> MACPLEKALDVMVSTFHKYSGKEGDKFKLNKSELKELLTRELPSFLGKRTDEAAFQK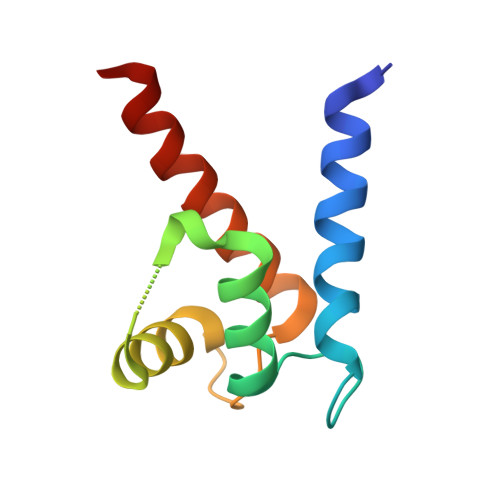LMSNLDSNRDNEVDFQEYCVFLSCIAMMCNEFFEGF> MTSITPVTLANCEDEPIHVPGAIQPHGALVTLRADGMVLAASENIQALLGFVASPGSYLTQEQVGPEVLRMLEEGLTGNGPWSNSVETRIGEHLFDVIGHSYKEVFYLEFEIRTADTLSITSFTLNAQRIIAQVQLHNDTASLLSNVTDELRRMTGYDRVMAYRFRHDDSGEVVAESRREDLESYLGQRYPASDIPAQARRLYIQNPIRLIADVAYTPMRVFPALNPETNESFDLSYSVLRSVSPIHCE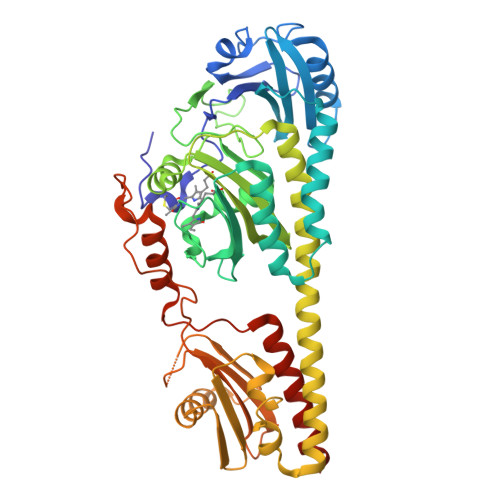YLTNMGVRASMSISIVVGGKLWGLFSCHHMSPKLIPYPVRMSFQIFSQVCSAIVERLEQGRIAELLRVSTERRLALARRARDADDLFGALAHPDDGIAALIPCDGALVMLGGRTLSIRGDFERQAGNVLQRLQRDPERDIYHTDNWPQPSEDSPDGGDCCGVLAIRFHRQESGWIFWFRHEEVHRIRWGGKPEKLLTIGPSGPRLTPRGSFEAWEEVVRGHSTPWSETDLAIAEKLRLDLMELCLNHALEHHHHHH2-(2,6-difluorophenyl)-4-(4-methoxyanilino)-5H-pyrrolo[3,4-d]pyrimidin-5-one 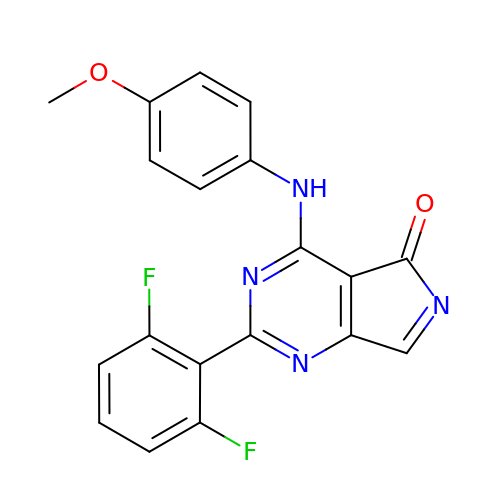| C19 H12 F2 N4 O2 | TWRUQHZKSONBRW-UHFFFAOYSA-N>[3x]GMA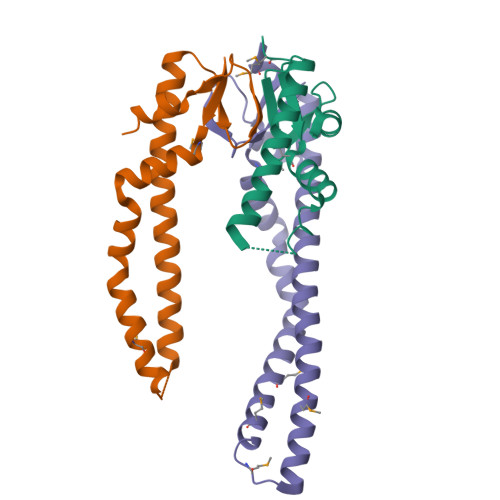DKIAIVNMGSLFQQVAQKTGVSNTLENEFKGRASELQRMETDLQAKMKKLQSMKAGSDRTKLEKDVMAQRQTFAQKAQAFEQDRARRSNEERGKLVTRIQTAVKSVANSQDIDLVVDANAVAYNSSDVKDITADVLKQVK> MADQTQEYTLSHTGGLLGSSKVTTASNQTAPQRETAIISFEVPRKFSEIEYVGQRDATRFVPRTTEEITGTANDDTVVQLQANIQ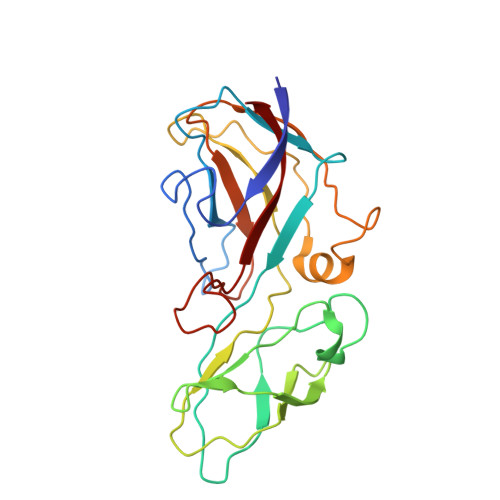PIAGEEDMADQDYPVVVAYNVTQGAQVEIADVNYATDEVTLATDPADGDTVKLWPIMGDGEVQFRLVNQFGQEEGRVYPWATPLYRWHDFPQLKRGREINLHGSVTWQENETVEVLLDAPQAITWEDADYPEGQYVSTFEQDVEITL> LGSGTTEDVSDLPVEEQLRRLQEERT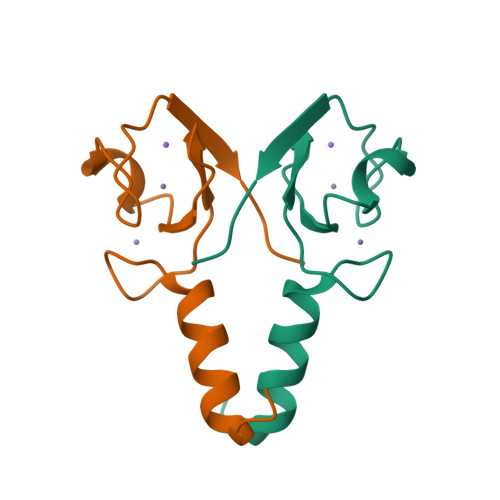CKVCMDKEVSIVFIPCGHLVVCKDCAPSLRKCPICRSTIKGTVRTFLS>[2x]MKKIEVYTQPDCPPCVIVKEFLK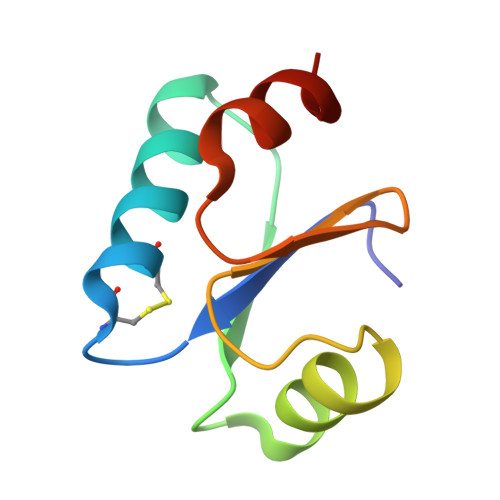HNNVAYEEFDVKKDAAARNRLLYDYDSYSTPTVVIDGEVVAGFQIEKLQQLLNIE> GHM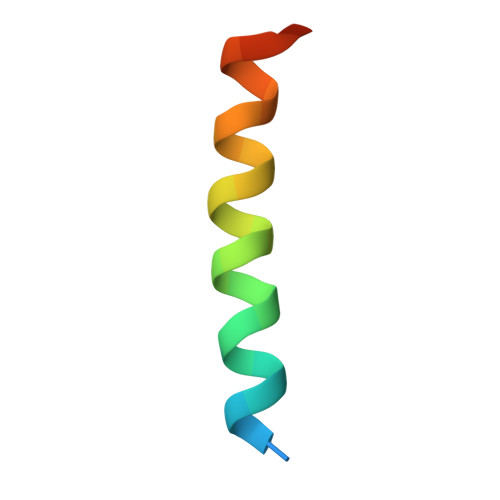EEIIHKLAMQLRHIGDNIDHRMVRED>MKVLVNHEQAYNVIINAINDAKKLTDYKTNNQWVSIQNVILGTHLTYRYILITGLLAKATDPRVNPLALQANAPVDGAYDARSLCHSVIVGKVEGPFLEGKLGASNEPFLNKPARYMLHSSDNPVRRGNDKVLQQLSIDILHAATTQTLAYEMLVIALYFTLQRTNRVITPNSINFDFHKIIYNIISHPCDGETCAIAAAISLHLLGEQRGWIIKAHPVNQAGSSSKEILDIDVYHDDIVFLSIEVKDKPFNYQDVNHAVSKASASGISKVIFLKGPRATNLDIDESLAIENAATKGVSLSFSDVMTFTTTCYALSP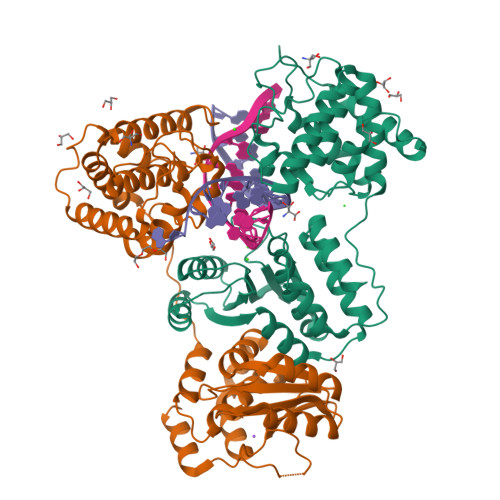LLSNDRIIDFINNTLKDIRAKDSTIEYIQSIFKN[2x]>MGSRLYDRRSIFDAVAQSNCQELESLLPFLQRSKKRLTDSEFKDPETGKTCLLKAMLNLHNGQNDTIALLLDVARKTDSLKQFVNASYTDSYYKGQTALHIAIERRNMTLVTLLVENGADVQAAANGDFFKKTKGRPGFYFGELPLSLAACTNQLAIVKFLLQNSWQPADISARDSVGNTVLHALVEVADNTVDNTKFVTSMYNEILILGAKLHPTLKLEEITNRKGLTPLALAASSGKIGVLAYILQREIHEPECRHLSRKFTEWAYGPVHSSLYDLSCIDTCEKNSVLEVIAYSSSETPNRHDMLLVEPLNRLLQDKWDRFVKRIFYFNFFVYCLYMIIFTAAAYYRPVEGLPPYKLKNTVGDYFRVTGEILSVSGGVYFFFRGIQYFLQRRPSLKSLFVDSYSEILFFVQSLFMLVSVVLYFSQRKEYVASMVFSLAMGWTNMLYYTRGFQQMGIYAVMIEKMILRDLCRFMFVYLVFLFGFSTAVVTLIEDGKYNSLYSTCLELFKFTIGMGDLEFTENYDFKAVFIILLLAYVILTYILLLNMLIALMGETVNKIAQESKNIWKLQRAITILDTEKSFLKCMRKAFRSGKLLQVGFTPDGKDDYRWCFRVDEVNWTTWNTNVGIINEDPG[2x]

The capsaicin- and heat-activated receptor, TRPV1, has served as a model for deciphering lipid modulation, which is relevant to understanding how pro-algesic agents enhance channel activity in the setting of inflammatory pain. Identification of a pocket within the TRPV1 transmembrane core has provided initial clues as to how phosphoinositide lipids bind to and regulate the channel. Here we show that this regulatory pocket in rat TRPV1 can accommodate diverse lipid species, including the inflammatory lipid lysophosphatidic acid, whose actions are determined by their specific modes of binding. We captured several states of TRPV1 ranging from channels in which the VBP is empty to those bearing different bioactive lipids, including distinct phosphoinositide species, brominated phosphoinositide analogs and a pro-algesic lipid, lysophosphatidic acid (LPA). Together, our data show how the VBP accommodates a range of bioactive lipids and how occupancy of the site corresponds to the structural status of the pore.

To resolve this question, we exploited our ability to generate TRPV1 protein with an empty vanilloid pocket, into which we introduced tetrabrominated analogs of PI or PIP2 (PI–Br4 and PIP2–Br4, respectively) as contrast-enhancing probes to distinguish these lipids from the other, unbrominated lipids in the nanodiscs. Previous work has established that brominated lipids are faithful analogs of the unsaturated lipids from which they are synthesized. In these high-resolution structures (2.2–2.4 Å resolution), we were able to identify the bromine atoms within the oleoyl tails of the lipids by visually comparing the resulting reconstructions against those previously determined for samples containing endogenous lipids. The well-resolved inositol headgroup of the bound lipids showed the expected differential location of phosphate moieties, most notably at the 4 and 5 positions for PIP2. Furthermore, conformations of both PI- and PIP2-reconstituted channels resemble the apo channel containing a native resident lipid. Together, these data demonstrate that the vanilloid site can accommodate PI or PIP2, where they act as negative regulatory factors to stabilize the closed state.N-[(3-carboxyphenoxy)acetyl]-L-glutamic acid | C14 H15 N O8 | 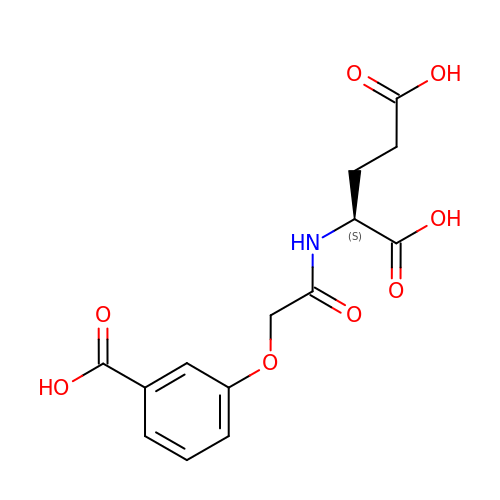ZYEJDCAIACBLPZ-JTQLQIEISA-N> MASGSCQGCEEDEETLKKLIVRLNNVQEGKQIETLVQILEDLLVFTYSERASKLFQGKNIHVPLLIVLDSYMRVASVQQVGWSLLCKLIEVCPGTMQSLMGPQDVGNDWEVLGVHQLILKMLTVHNASVNLSVIGLKTLDLLLTSGKITLLILDEESDIFMLIFDAMHSFPANDEVQKLGCKALHVLFERVSEEQLTEFVENKDYMILLSALTNFKDEEEIVLHVLHCLHSLAIPCNNVEVLMSGNVRCYNIVVEAMKAFPMSERIQEVSCCLLHRLTLGNFFNILVLNEVHEFVVKAVQQYPENAALQISALSCLALLTETIFLNQDLEEKNENQENDDEGEEDKLFWLEACYKALTWHRKNKHVQEAACWALNNLLMYQNSLHEKIGDEDGHFPAHREVMLSMLMHSSSKEVFQASANALSTLLEQNVNFRKILLSKGIHLNVLELMQKHIHSPEVAESGCKMLNHLFEGSNTSLDIMAAVVPKILTVMKRHETSLPVQLEALRAILHFIVPGMPEESREDTEFHHKLNMVKKQCFKNDIHKLVLAALNRFIGNPGIQKCGLKVISSIVHFPDALEMLSLEGAMDSVLHTLQMYPDDQEIQCLGLSLIGYLITKKNVFIGTGHLLAKILVSSLYRFKDVAEIQTKGFQTILAILKLSASFSKLLVHHSFDLVIFHQMSSNIMEQKDQQFLNLCCKCFAKVAMDDYLKNVMLERACDQNNSIMVECLLLLGADANQAKEGSSLICQVCEKESSPKLVELLLNSGSREQDVRKALTISIGKGDSQIISLLLRRLALDVANNSICLGGFCIGKVEPSWLGPLFPDKTSNLRKQTNIASTLARMVIRYQMKSAVEEGTASGSDGNFSEDVLSKFDEWTFIPDSSMDSVFAQSDDLDSEGSEGSFLVKKKSNSISVGEFYRDAVLQRCSPNLQRHSNSLGPIFDHEDLLKRKRKILSSDDSLRSSKLQSHMRHSDSISSLASEREYITSLDLSANELRDIDALSQKCCISVHLEHLEKLELHQNALTSFPQQLCETLKSLTHLDLHSNKFTSFPSYLLKMSCIANLDVSRNDIGPSVVLDPTVKCPTLKQFNLSYNQLSFVPENLTDVVEKLEQLILEGNKISGICSPLRLKELKILNLSKNHISSLSENFLEACPKVESFSARMNFLAAMPFLPPSMTILKLSQNKFSCIPEAILNLPHLRSLDMSSNDIQYLPGPAHWKSLNLRELLFSHNQISILDLSEKAYLWSRVEKLHLSHNKLKEIPPEIGCLENLTSLDVSYNLELRSFPNEMGKLSKIWDLPLDELHLNFDFKHIGCKAKDIIRFLQQRLKKAVPYNRMKLMIVGNTGSGKTTLLQQLMKTKKSDLGMQSATVGIDVKDWPIQIRDKRKRDLVLNVWDFAGREEFYSTHPHFMTQRALYLAVYDLSKGQAEVDAMKPWLFNIKARASSSPVILVGTHLDVSDEKQRKACMSKITKELLNKRGFPAIRDYHFVNATEESDALAKLRKTIINESLNFKIRDQLVVGQLIPDCYVELEKIILSERKNVPIEFPVIDRKRLLQLVRENQLQLDENELPHAVHFLNESGVLLHFQDPALQLSDLYFVEPKWLCKIMAQILTVKVEGCPKHPKGIISRRDVEKFLSKKRKFPKNYMSQYF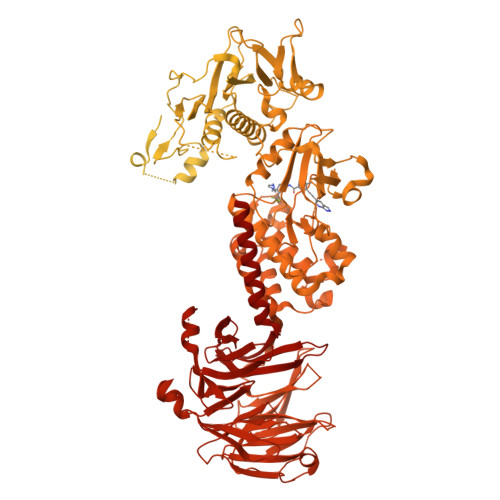KLLEKFQIALPIGEEYLLVPSSLSDHRPVIELPHCENSEIIIRLYEMPYFPMGFWSRLINRLLEISPYMLSGRERALRPNRMYWRQGIYLNWSPEAYCLVGSEVLDNHPESFLKITVPSCRKGCILLGQVVDHIDSLMEEWFPGLLEIDICGEGETLLKKWALYSFNDGEEHQKILLDDLMKKAEEGDLLVNPDQPRLTIPISQIAPDLILADLPRNIMLNNDELEFEQAPEFLLGDGSFGSVYRAAYEGEEVAVKIFNKHTSLRLLRQELVVLCHLHHPSLISLLAAGIRPRMLVMELASKGSLDRLLQQDKASLTRTLQHRIALHVADGLRYLHSAMIIYRDLKPHNVLLFTLYPNAAIIAKIADYGIAQYCCRMGIKTSEGTPGFRAPEVARGNVIYNQQADVYSFGLLLYDILTTGGRIVEGLKFPNEFDELEIQGKLPDPVKEYGCAPWPMVEKLIKQCLKENPQERPTSAQVFDILNSAELVCLTRRILLPKNVIVECMVATHHNSRNASIWLGCGHTDRGQLSFLDLNTEGYTSEEVADSRILCLALVHLPVEKESWIVSGTQSGTLLVINTEDGKKRHTLEKMTDSVTCLYCNSFSKQSKQKNFLLVGTADGKLAIFEDKTVKLKGAAPLKILNIGNVSTPLMCLSESTNSTERNVMWGGCGTKIFSFSNDFTIQKLIETRTSQLFSYAAFSDSNIITVVVDTALYIAKQNSPVVEVWDKKTEKLCGLIDCVHFLREVMVKENKESKHKMSYSGRVKTLCLQKNTALWIGTGGGHILLLDLSTRRLIRVIYNFCNSVRVMMTAQLGSLKNVMLVLGYNRKNTEGTQKQKEIQSCLTVWDINLPHEVQNLEKHIEVRKELAEKMRRTSVE>MVATPVKQKYDIKDISLAPQGRQRIEWAAREMPVLKQIRERFAQEKPFAGIRLVACCHVTTETANLAIALHAGGADSLLIASNPLSTQDDVAACLVADYGIPVYAIKGEDNETYHRHVQIALDHRPNIIIDDGSDVVATLVQERQHQLSDIIGTTEETTTGIVRLRAMFNDGVLTFPAMNVNDADTKHFYDNRYGTGQSTLDGIIRATNILLAGKTIVVAGYGWCGKGVAMRAKGMGADVIVTEISPVPAIEAAMDGFRVMPMAEAAHQGDIFITVTGNKHVIRPEHFAVMKDGAIVCNSGHFDIEIDLKSLKEQAKEVKEVRNFTEQYILPNGKSIIVIGEGRLVNLAAATGHPSAVMDMSFANQALACEHLVKNKGQLEPGMHSIPVEVDQEIARLKLQAMGIAIDSLTPEQ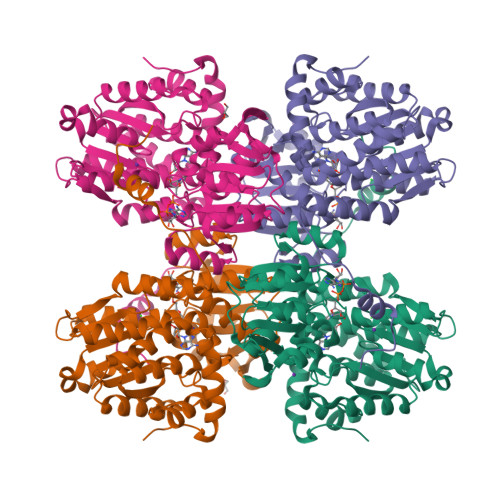VEYINSWASGT[2x]>MTEETISQAVPPVRDWPAVDLPGSDFDPVLTELMREGPVTRISLPNGEGWAWLVTRHDDVRLVTNDPRFGREAVMDRQVTRLAPHFRPARGAVGFLDPPDHTRLRRSVAAAFTARGVERVRERSRGMLDELVDAMLRAGPPADLTEAVLSPFPIAVICELMGVPATDRHSMHTWTQLILSSSHGA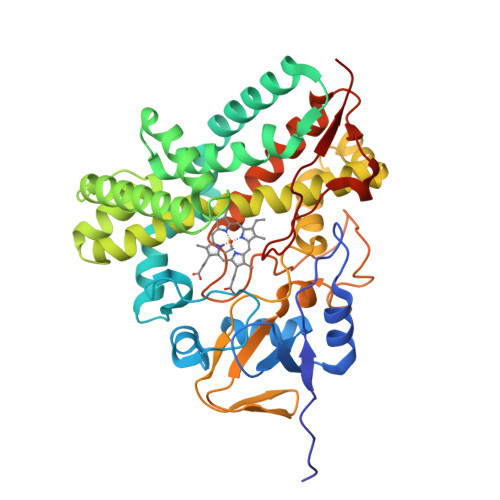EVSERAKNEMNAYFSDLIGLRSDSAGEDVTSLLGAAVGRDEITLSEAVGLAVLLQIGGEAVTNNSGQMFHLLLSRPELAERLRSEPEIRPRAIDELLRWIPHRNAVGLSRIALEDVEIKGVRIRAGDAVYVSYLAANRDPEVFPDPDRIDFERSPNPHVSFGFGPHYCPGGMLARLESELLVDAVLDRVPGLKLAVAPEDVPFKKGALIRGPEALPVTWHHHHHH[2x]> MYEAIGHRVEDGVAEITIKLPRHRNALSVKAMQEVTDALNRAEEDDSVGAVMITGAEDAFCAGFYLREIPLDKGVAGVRDHFRIAALWWHQMIHKIIRVKRPVLAAINGVAAGGGLGISLASDMAICADSAKFVCAWHTIGIGNDTATSYSLARI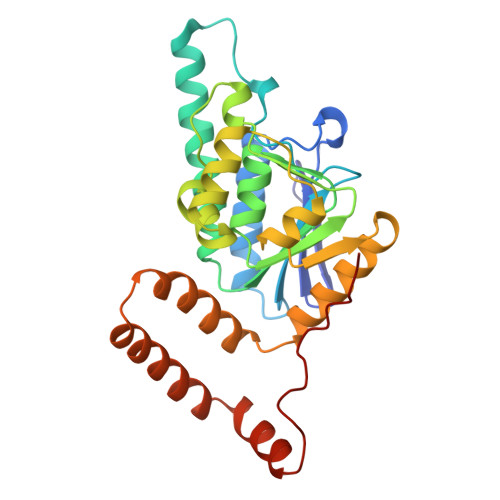VGMRRAMELMLTNRTLYPEEAKDWGLVSRVYPKDEFREVAWKVARELAAAPTHLQVMAKERFHAGWMQPVEECTEFEIQNVIASVTHPHFMPCLTRFLDGHRADRPQVELPAGV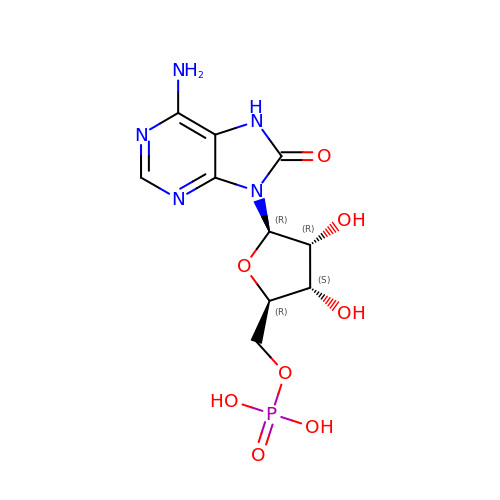[(2R,3S,4R,5R)-5-(6-azanyl-8-oxo-7H-purin-9-yl)-3,4-dihydroxy-oxolan-2-yl]methyl dihydrogen phosphate | C10 H14 N5 O8 P | JPZDUYBDBSYCDZ-UUOKFMHZSA-N> MTDYTDHLATGCTTLARCYILTRRDGVVMGFTDHDRDIDLDGTRCAAGAALDASTAARSLGITPDDMDAGGALSADAITEADLRAGRYDGAQVEVWEVNWTDPAVRGRLGVYTIGQVERGPLAFRAELRTRPALWNRPEGRIHTALCDVDRLGDHRCKLALGPWQSAATVIEADGADLIVSGLDETASNIFDRGVLDWTGGANAGTGSDIRVARPVAGGVRVSLWSAPPFPITAGDTANATVGCDRTADTCRNRF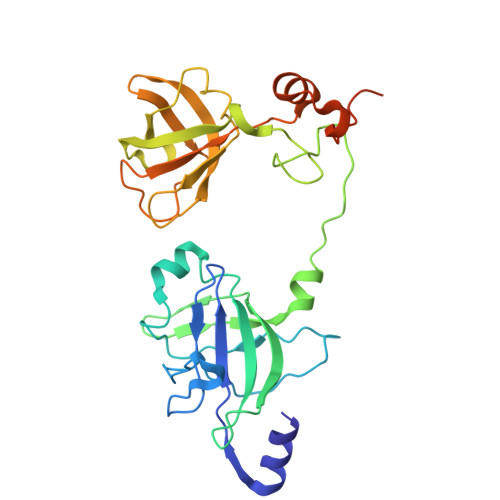DNLANFRGFPLMPGESFISEYARPGDPDQSGGSRYD>[2x]MDTTDIKPVRPAINLQQPPFVVGRLLRTVQDEERGFTLPGAGKLADLFESTALKLAQSARINTWLVKGTSVDDAFLKLELNTAGSRIFENPKLLTWAVYVTKVEKQNPEEIIL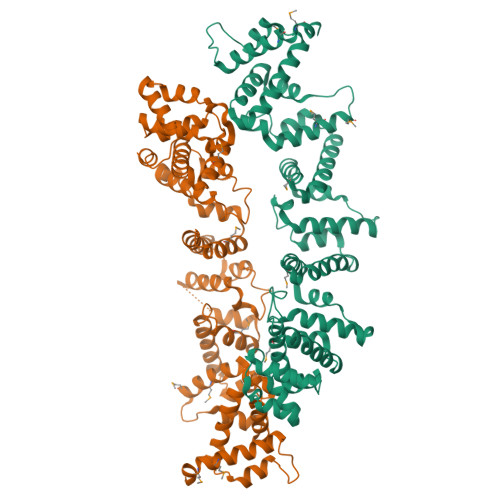AKLSKQFTEGSLAKMIASAKLDSKTEGLATILQAQQRQVWVDAGKSSDEVFKLLQLDEAGTKLFKNQQFSTWTSFVDAFNRKYPEKAVSIFSKLAKTYDGFTLWKMLEAAKKVPKTEIIASKLQAQQIDAWLDAGKSTDEVFNLLKLQRTGDKLFKNSQFLTWVSYVEKFNKKDPDQAIAIFSKLAGVYDQVTLSSMLEAAKHVPSTKRIASYLQGQQNQHWLADGKSTDDIFKLLKLNTPSPENLIDPRLDAWTSFMRAFNMANEGKETTLIATLTTHYKDRGLAQLLQEGTKFASTKKIAEELQTAQFARWLQLGKTEDDIFALLKLKLTTPTTDPEAIVFYQYKLFMDAHMKLAAA2,2-bis(fluoranyl)ethyl 4-(2,3-dihydroindol-1-yl)-4-oxidanylidene-butanoate | C14 H15 F2 N O3 | 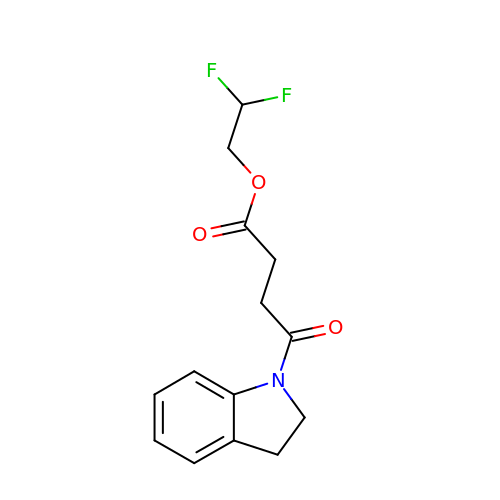ZBGADGOMZKMKIY-UHFFFAOYSA-N> SMPAISMPQKSFNATAERGEEMTFSCRASGSPEPAISWFRNGKLIEENEKYILKGSNTELTVRNIINSDGGPYVCRATNKAGEDEKQAFLQVFVQPHIIQLKNET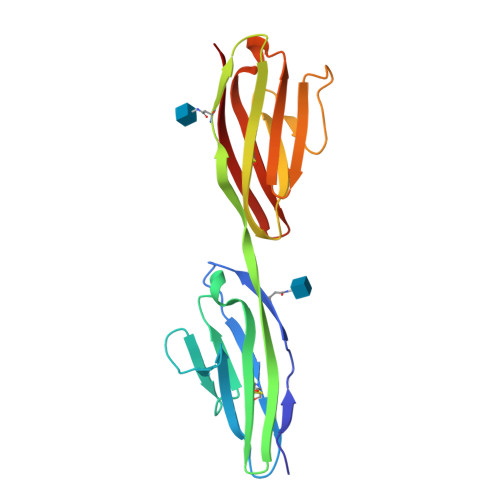TYENGQVTLVCDAEGEPIPEITWKRAVDGFTFTEGDKSLDGRIEVKGQHGSSSLHIKDVKLSDSGRYDCEAASRIGGHQKSMYLDIE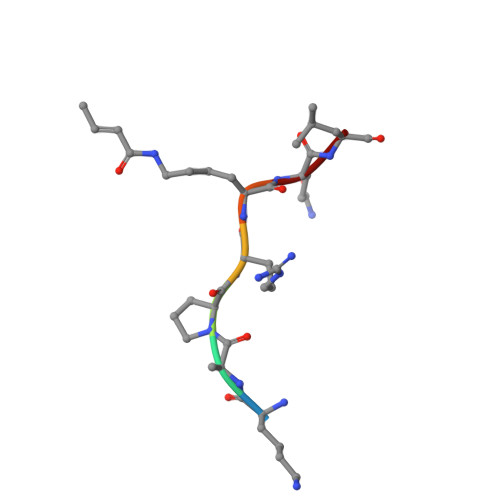> KAPRXQL>GSHMMGAKMAESLRLTCLACGQANKVPSDRLAAGPKCGICGAGLITGKVAGIDPAILARA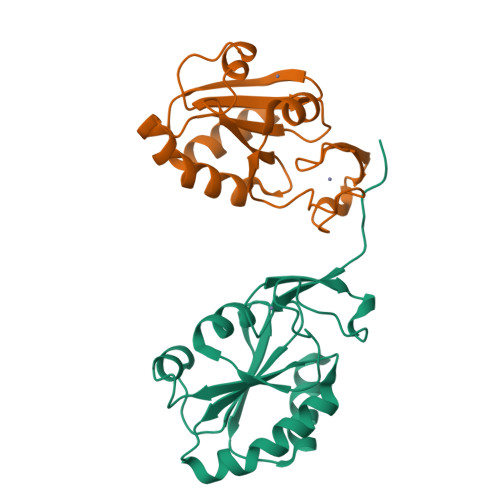ERDDLPLLVDFWAPWCGPCRQMAPQFQAAAATLAGQVRLAKIDTQAHPAVAGRHRIQGIPAFILFHKGRELARAAGARPASELVGFVRGKLGARA[2x]>[8x]MSLTAPVKLAIVFYSSTGTGYAMAQEAAEAGRAAGAE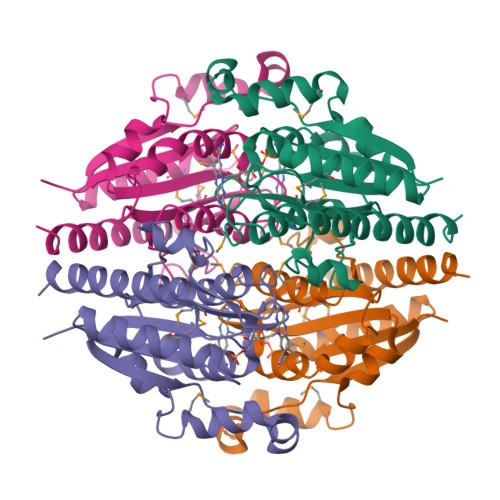VRLLKVRETAPQDVIDGQDAWKANIEAMKDVPEATPADLEWAEAIVFSSPTRFGGATSQMRAFIDTLGGLWSSGKLANKTFSAMTSAQNVNGGQETTLQTLYMTAMHWGAVLTPPGYTDEVIFKSGGNPYGASVTANGQPLLENDRASIRHQVRRQVELTAKLLEGGSHHHHHH Methylation on the ε-amine of the lysine side chain is catalyzed by a family of approximately 60 lysine methyltransferase (KMT) enzymes. SMYD2 has been reported to monomethylate or dimethylate histone H3 (H3K4me1 and H3K36me2), p53 (K370me1), RB (K860me1), MAPKAPK3 (K355me1), and numerous other proteins. In addition, small-molecule inhibitors for a variety of clinical indications are currently under development for SMYD2 (21). These therapeutic efforts are primarily based on the biological connection that SMYD2 methylates the tumor suppressor protein p53, leading to inhibition of p53 function.

K-OPL analysis of SMYD2 substrate selectivity revealed that the optimal substrate is not found in the human proteome (WKLKSKR) due to the tryptophan in the P−3 position. Replacement of a substrate’s target lysine with Nle has been previously used as an inhibitory strategy for KMTs. As a proof of concept for K-OPL–guided discovery of KMT inhibitors, we synthesized Nle-containing peptides based on the optimal SMYD2 substrate and found that the Nle derivative of WKLKSKR inhibited SMYD2 methylation of PER2. The unresolved amino acid in the P−3 position was modeled, and all-atom MD simulations of this structure in complex with the peptides used for in vitro KMT assays allowed us to evaluate the dynamics of SMYD2-substrate interactions. MD simulations showed that the tryptophan settles in a hydrophobic pocket near the SMYD2 active site, and a recently found small-molecule inhibitor of SMYD2 contains a bulky aromatic group that also binds in this same pocket. Thus, the K-OPL screening platform identified a SMYD2-substrate interaction that would never have been found through the analysis of previously identified SMYD2 substrates. Overall, these results suggest that optimal substrates identified by K-OPL screens can serve as scaffolds for further optimization toward more potent inhibitors.

>[2x]GLGGLERFCSPGKGRGLRALQPFQVGDLLFSCPAYAYVLTVNERGNHCEYCFTRKEGLSKCGRCKQAFYCNVECQKEDWPMHKLECSPMVVFGENWNPSETVRLTARILAKQKIHPERTPSEKLLAVKEFESHLDKLDNEKKDLIQSDIAALHHFYSKHLEFPDNDSLVVLFAQVNCNGFTIEDEELSHLGSAIFPDVALMNHSCCPNVIVTYKGTLAEVRAVQEIKPGEEVFTSYIDLLYPTEDRNDRLRDSYFFTCECQECTTKDKDKAKVEIRKLSDPPKAEAIRDMVRYARNVIEEFRRAKHYKSPSELLEICELSQEKMSSVFEDSNVYMLHMMYQAMGVCLYMQDWEGALQYGQKIIKPYSKHYPLYSLNVASMWLKLGRLYMGLEHKAAGEKALKKAIAIMEVAHGKDHPYISEIKQEIESH;>KLLSKRG[2x]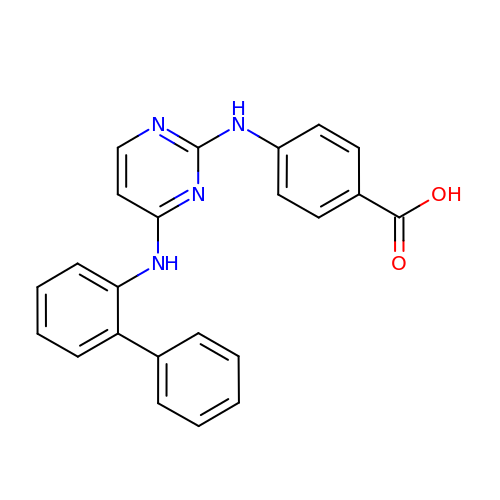4-{[4-(biphenyl-2-ylamino)pyrimidin-2-yl]amino}benzoic acid | C23 H18 N4 O2 | RSUKUXYTJJCQKG-UHFFFAOYSA-N> GSSHHHHHHTDPVIAQKAPYPVTVEAGKTYHWCACGRSKAQPFCDGSHKGTGLAPVAYTPDKAGTAYFCGCKASKAPPLCDGTHKTL

The recently discovered CDGSH iron-sulfur domains (CISDs) are characterized by one or two highly conserved 17-residue CDGSH motifs with a consensus sequence of [ΦCXCXX(S/T)XXXPΦCDG(S/T/A)H], where Φ and X are a hydrophobic or any residue, respectively. The [2Fe-2S] cluster is coordinated with three cysteine residues and one histidine residue in the CDGSH motif. We synthesized genes for a type 3 CISD (PcCISD) from Pyrobaculum calidifontis, which is a hyperthermophilic archaeon, a type 4 CISD (RsCISD) from Ralstonia solanacearum, which is a soil-born plant pathogenic bacterium, and a type 6 CISD (MmCISD) from Magnetospirillum magneticum, which is an aquatic alphabacterium that utilizes iron reduction to derive energy. The four CISD structures display striking similarity in their overall appearance, with dual iron-sulfur binding modules and a β-sandwich dimerization module.

The MmCISD structure was determined by single-wavelength anomalous dispersion (SAD) using the anomalous signal from the bound iron. The MmCISD structure is monomeric, with each of its two CDGSH motifs binding a [2Fe-2S] cluster. The pear-shaped structure consists of two iron-sulfur binding modules at the base and a compact β-sandwich on the top. The structure is composed of mainly loop regions (L1 though L5) interspersed by four short β-strands (β1 though β4) with a topology of L1-β1-L2-β2-L3-β3-L4-β4-L5. One [2Fe-2S] cluster is coordinated by Cys25, Cys27, Cys36 and His40 in the N-terminal CDGSH motif in loop L3, whereas the other [2Fe-2S] cluster is coordinated by Cys61, Cys63, Cys72 and His76 in the C-terminal CDGSH motif in loop L5, as predicted. The monomeric structure of MmCISD displays an internal pseudo 2-fold symmetry and bears remarkable similarity to other homodimeric CISD structures. The N-terminal half (L1-β1-L2-β2-L3) is related to the C-terminal half (β3-L4-β4-L5) by a pseudo dyad axis passing through the center of the structure. The two iron-sulfur binding modules pack back-to-back with a polar interface. The completely buried Lys64 plays a key role in bridging the two iron-sulfur binding modules. The side chain amino group of Lys64 forms three hydrogen bonds simultaneously with the backbone carbonyl oxygen of Cys61 and Cys25 and the side chain carbonyl oxygen of Gln33.Src homology 3 (SH3)-domain growth factor receptor-bound 2-like (endophilin) interacting protein 1 (SGIP1) and its splicing variant, SGIP1α, are brain-specific homologs of FCHo1/FCHo2. The μHDs of SGIP1 and SGIP1α, which are identical to each other, are highly homologous to those of FCHo1/FCHo2. The μHD of SGIP1/SGIP1α also binds to the DPF motif-rich region of Eps1519. Thus, the SGIP1/FCHo1/FCHo2 μHD is a domain designed for recognizing the locally ordered structure formed by the two consecutive DPF motifs.

We next crystallized the complex between the SGIP1 μHD and two short μHD-binding Eps15 fragments containing two DPF motifs derived from the high-affinity μHD-binding site, Eps15-640–649 and Eps15-645–654. In the two structures, the two DPF motifs are recognized by a continuous cleft on the μHD. The two DPF motifs in the two structures adopt type-I β-turn conformations, and each is stabilized by two sequence-specific intramotif interactions. In our complex structures, the two DPF motifs are intimately packed against each other through hydrophobic interactions between the side chains of Phe in the N-terminal DPF motif and Pro in the C-terminal DPF motif. This arrangement of the DPF motifs brings the hydrophobic side chains of all of the Pro and Phe residues of the two DPF motifs together on one side, allowing their extensive recognition by the continuous hydrophobic cleft of the μHD. Two conserved Ala residues, Ala563 and Ala565, of SGIP1 are located at the bottom of this recognition cleft. Ala563 contacts the side chains of Phe in the N-terminal DPF motif and Pro in the C-terminal DPF motif, while Ala565 contacts the side chains of Pro and Phe in the N-terminal DPF motif. In the two structures, the two DPF motifs bind to the same recognition cleft on the μHD. However, the positions of the C-terminal DPF motif relative to the recognition cleft slightly differ between the two structures, probably due to differences in the lengths and the amino acid sequences of the linker region between the two DPF motifs. Nevertheless, the key interactions for DPF motif recognition by the μHD are essentially conserved in the two structures (see below).

> GPLGSLTMGAQDTLPVAAAFTETVNAYFKGADPSKCIVKITGEMVLSFPAGITRHFANNPSPAALTFRVINFSRLEHVLPNPQLLCCDNTQNDANTKEFWVNMPNLMTHLKKVSEQKPQATYYNVDMLKYQVSAQGIQSTPLNLAVNWRCEPSSTDLRIDYKYNTDAMTTAVALNNVQFLVPIDGGVTKLQAVLPPAVWNAEQQRILWKIPDISQKSENGGVGSLLARFQLSEGPSKPSPLVVQFTSEGSTLSGCDIELVGAGYRFSLIKKRFAAGKYLADN;> YDPFKGSDPFA> GSASAPTLFPLVSCENSPSDTSSVAVGCLAQDFLPDSITFSWKYKNNSDISSTRGFPSVLRGGKYAATSQVLLPSKDVMQGTDEHVVCKVQHPNGNKEKNVPLPVIAELPPKVSVFVPPRDGFFGNPRKSKLICQATGFSPRQIQVSWLREGKQVGSGVTTDQVQAEAKESGPTTYKVTSTLTIKESDWLGQSMFTCRVDHRGLT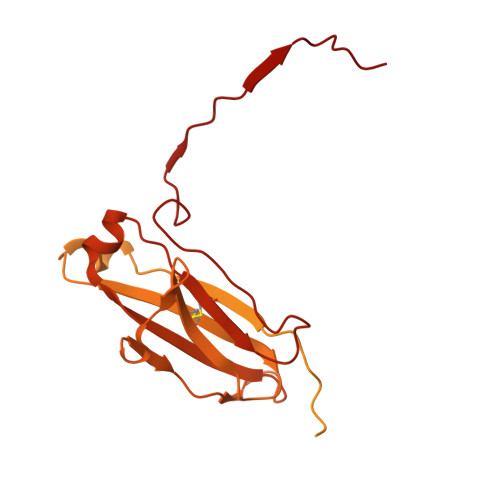FQQNASSMCVPDQDTAIRVFAIPPSFASIFLTKSTKLTCLVTDLTTYDSVTISWTRQNGEAVKTHTNISESHPNATFSAVGEASICEDDWNSGERFTCTVTHTDLPSPLKQTISRPKGVALHRPDVYLLPPAREQLNLRESATITCLVTGFSPADVFVQWMQRGQPLSPEKYVTSAPMPEPQAPGRYFAHSILTVSEEEWNTGETYTCVVAHEALPNRVTERTVDKSTGKPTLYNVSLVMSDTAGTCY>MRLEIPNHTERFGVVRLHEVQRILELDSGRVRDESPAVGLRRLDDADLRDVLEQTAIVVPTRNERLKLLEGVLSGIPHEALILVASNSSPDRFQMERDLLEEFAHLTERPALIFHQKDPALAEALRAGGYPHPIGEDGLVRSGKAEGMILALVFAALSGRRYVGFIDADNYFPGAVWEYVRAYAAGFLMAKTPFAMVRILWRYKPKLTEDEGVVFRRYGRVSERNNRALNQLIGGVSGFETDVVKTANAGEHAMSLGLALRLPLASGYAVEPQELVSLLELYGGVFPLEDEEVLQHGVEIFQI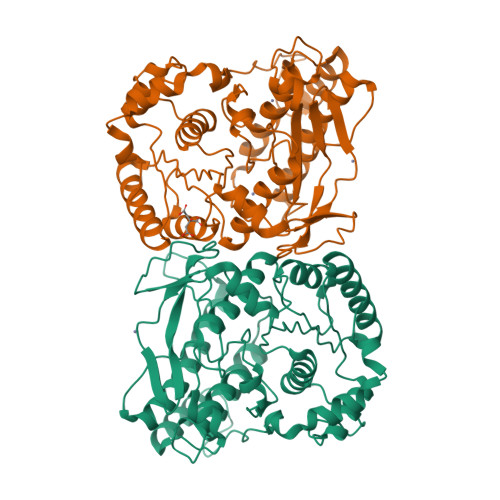ETRNPHLHENKGDEHIRDMLLACLATVYHSKLATEEVRQSVLEELQAAGALAPGEEPPPPVLYPPLSSLDLQAVRKALRGHFSRFRVP[2x]tert-butyl 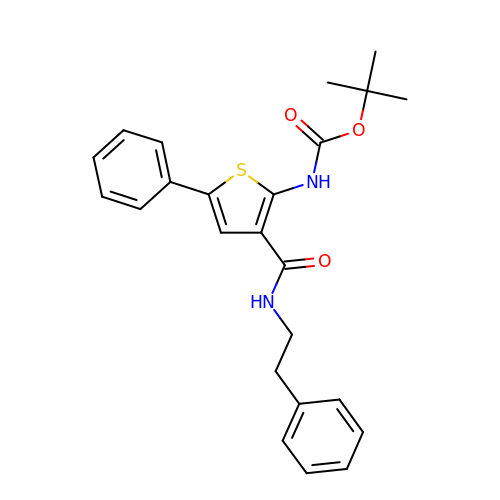N-[5-phenyl-3-(2-phenylethylcarbamoyl)thiophen-2-yl]carbamate | C24 H26 N2 O3 S | RNVBPELOZDZKOV-UHFFFAOYSA-N>[2x]RFLKVKNWETDVVLTDTLHLKSTLETGCTEHICMGSIVLPSQHTRKPEDVRTKDQLFPLAKEFLDQYYSSIKRFGSKAHM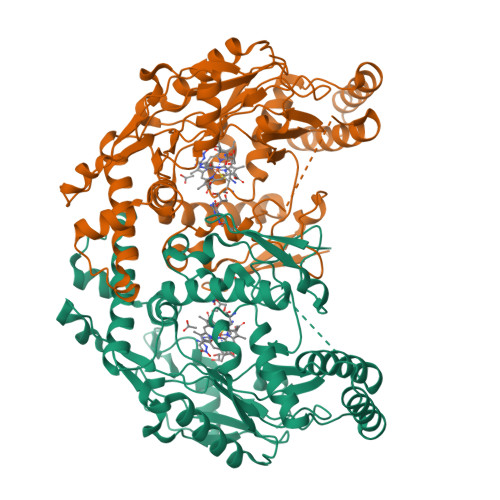DRLEEVNKEIESTSTYQLKDTELIYGAKHAWRNASRCVGRIQWSKLQVFDARDCTTAHGMFNYICNHVKYATNKGNLRSAITIFPQRTDGKHDFRVWNSQLIRYAGYKQPDGSTLGDPANVQFTEICIQQGWKAPRGRFDVLPLLLQANGNDPELFQIPPELVLEVPIRHPKFDWFKDLGLKWYGLPAVSNMLLEIGGLEFSACPFSGWYMGTEIGVRNYCDNSRYNILEEVAKKMDLDMRKTSSLWKDQALVEINIAVLYSFQSDKVTIVDHHSATESFIKHMENEYRCRGGCPADWVWIVPPMSGSITPVFHQEMLNYRLTPSFEYQPDPWNTHVWKG> MAHHHHHHDDDDKIRTLPGEGTQVHPRAPLLQILKVAGAQEEVFTVKEVMHYLGQYIMMKQLYDKQRQHIVHCHDDPLGELLEV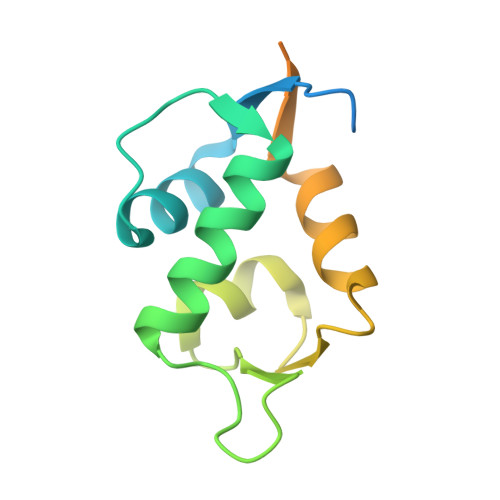GSFSVKNPSPLYEMLKRNLVILNNSDAAKNLSVGKDSNESPSEDPGQVSSGSINSA Hyp-1 is a 165-residue pathogenesis-related class 10 (PR-10) protein from the medicinal herb St John’s wort (Hypericum perforatum). The mystery shrouding the function of PR-10 proteins is in contrast to their comprehensive structural characterization, which reveals an almost hollow molecular core surrounded by a seven-stranded antiparallel β-sheet gripped around a long α-helix (α3) supported at the C-terminus by a fork of two shorter helices. This characteristic fold, termed the PR-10 fold (or the Bet v 1 fold after birch pollen allergen, which was the first PR-10 protein to have its crystal structure solved) strongly suggests the binding/storage of hydrophobic ligands. Hyp-1 has been postulated to catalyze the oxidative coupling of emodin to hypericin, the main pharmacological ingredient of St John’s wort, although this enzymatic activity has been questioned.

Large single crystals of a Hyp-1–ANS complex were obtained by co-crystallization with an eightfold molar excess of the ligand. The maps show excellent electron density for either one, two or three internal ANS molecules (at sites designated 1, 2 and 3) per Hyp-1 protein and 29 interstitial ANS molecules. Two ligands are bound in internal chambers (sites 1 and 2) and one in a deep surface pocket (site 3) formed by residues Lys33 and Tyr150. Sites 1, 2 and 3 are occupied in 22, 25 and 13, respectively, of the 28 protein molecules in the asymmetric unit. The structure shows three clearly defined and separated ligand-binding sites, and the fact that the complex stoichiometry can be 1:1, 1:2 or 1:3 has to be taken into account as a complication when studying the kinetics and stoichiometry of PR-10–ligand complexes using ANS displacement fluorescence. Fortunately, the structure shows that there is no direct interaction between the fluorescing species to further complicate the spectra. The Hyp-1 molecules are arranged into dimers through intermolecular β-sheet formation between β1–β1 strands, although the protein is monomeric in solution. Seven of these dimers have the same orientation and nearly equal repetitive spacing along the c axis, while the remaining seven are their copies through a noncrystallographic 21 axis in the c direction. Rigid-body refinement of the 28 copies of the protein molecule in the C2 solution confirmed that this solution does not obey any higher symmetry, though it is pseudo-symmetric with pseudo-tetragonal symmetry. The final electron-density maps are of very good quality, showing unambiguously the main-chain trace of all 28 independent protein molecules (A, B, … Z, a, b), clear conformations for most side chains and good density for all copies of the C-terminal helix α3, which is often disordered in PR-10 structures.

>[28x]GIDPFTMAAYTIVKEEESPIAPHRLFKALVLERHQVLVKAQPHVFKSGEIIEGDGGVGTVTKITFVDGHPLTYMLHKFDEIDAANFYCKYTLFEGDVLRDNIEKVVYEVKLEAVGGGSKGKITVTYHPKPGCTVNEEEVKIGEKKAYEFYKQVEEYLAANPEVFA4-HYDROXY-1,2,5-OXADIAZOLE-3-CARBOXYLIC 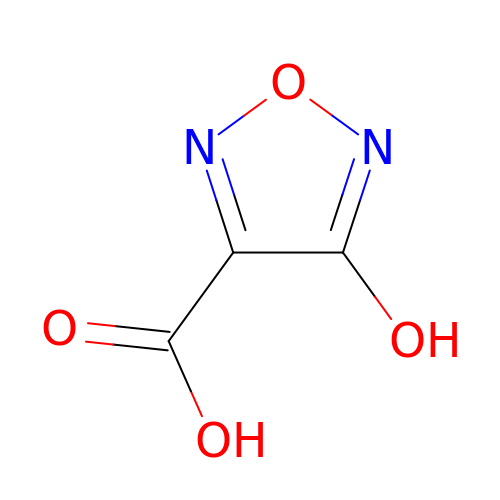ACID | C3 H2 N2 O4 | IBRWUZLLHSXPKL-UHFFFAOYSA-N> MASMTGGQQMGRDEAGI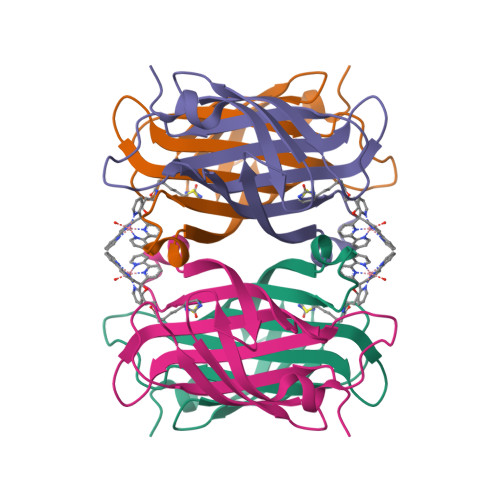TGTWYNQLGSTFIVTAGADGALTGTYESAVGNAESRYVLTGRYDSAPATDGSGTALGWTVAWKNNYRNAHSATTWSGQYVGGAEARINTQWLLTSGTTEANAWASTLVGHDTFTKVKPSAASIDAAKKAGVNNGNPLDAVQQ>[2x]GSHMSFRDNLKVYIESPESYKNVIYYD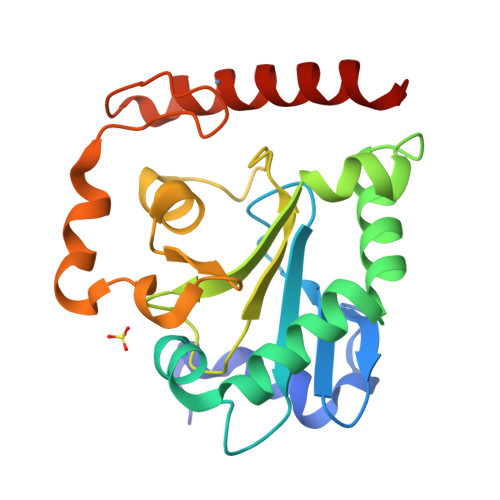DDVVLVRDMFPKSKMHLLLMTRDPHLTHVHPLEIMMKHRSLVEKLVSYVQGDLSGLIFDEARNCLSQQLTNEALCNYIKVGFHAGPSMNNLHLHIMTLDHVSPSLKNSAHYISFTSPFFVKIDTPTSNLPTRGTLTSLFQEDLKCWRCGETFGRHFTKLKAHLQEEYDDWLDKSVSM>GPHMASMDENEFDNQRENKAVARVIISFLKYEEYALKEIYNLRVKKWASISDRQKDMVPNYTKYLANLKAAIIENGKFFRSVAEYALQSISFEPGEIVQPNDLDMSKTCSLLTQVYREWSAEAISERNCLNSRLVPFLKTLSPPKADILIPGCGTGRLLVDLSRMGYNCEGNEFSYHMLLVSQYMLNAGLLQNQIIIYPFIHCFSHWKKIEDQLSPIKVPDIEAWSSNKGMGSMSICAGSFVDCYGRNQGTKISSHYTFSRRMQLSRAKAENSKDVVVTNFFIDTGSNILDYLDTIGHVLKPGGIWCNFGPLLYHFENDHGVETTYEVNPYSGFQDKINDYTPLMGLELSSDDIISIATNHLDFELIRRESGILCGYGRYAGPESCAMPGYMCHYWILKSNPTNES[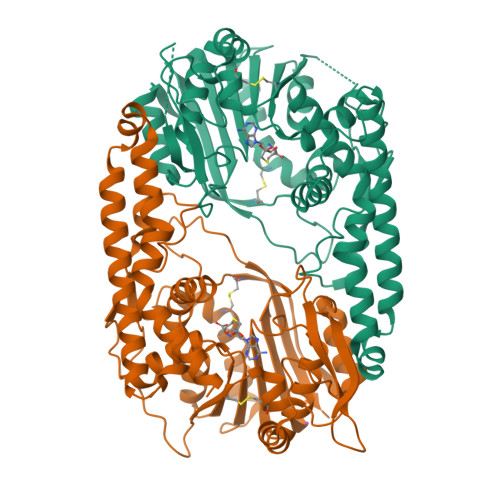2x]> GSHMPALPIDQEFDCERFRADIRATAAAIGAPIAHRLTDTVLEAFRDNFAQGATLWKTTSQPGDQLSYRFFSRLKMDTVSRAIDAGLLDAAHPTLAVVDAWSSLYGGAPVQSGDFDAGRGMAKTWLYFGGLRPAEDILTVPALPASVQARLKDFLALGLAHVRFAAVDWR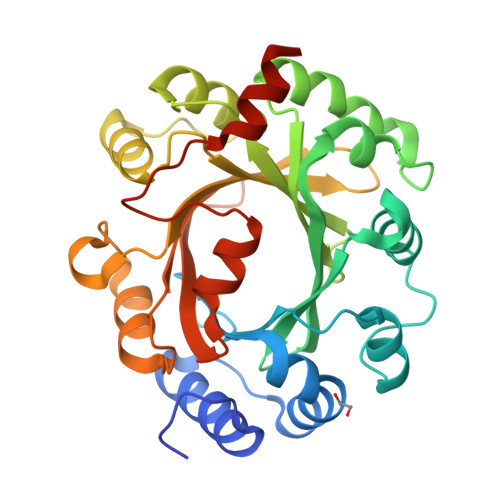HHSANVYFRGKGPLDTVQFARIHALSGSTPPAAHVVEEVLAYMPEDYSVAITLDLHSGDIERVCFYALKVPKNALPRIPTRIARFLEVAPSHDVEECNVIGWSFGRSGDYVKAERSYTGNMAEILAGWNCFFHGEEGRDHDLRALHQHTESTMGGAR>MSSG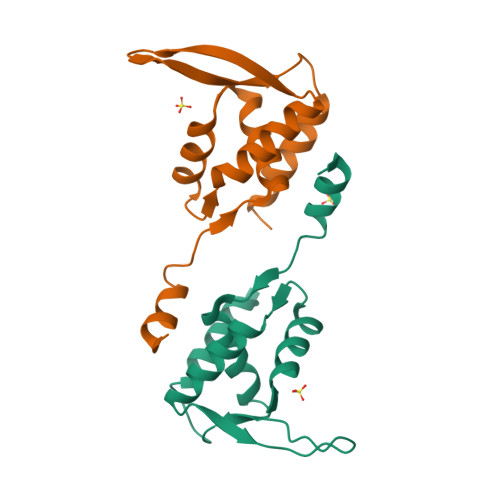VAAPQPSSCVPSRVSVLSMDFEDIYRFFQDPPPHYLSKELAVCYVLAVLRHEDSYGTELIQHLETHWPNYRLSDTVLYTALKFLEDEQIISGYWKKVEGRGRPRRMYQLAQANDDRSRDLAQLWERYLSSSAATDRQLIPVEAR[4x]>[6x]GSHMGTEDLKYSLERLREILERLEENPSEKQIVEAIRAIVENNAQIV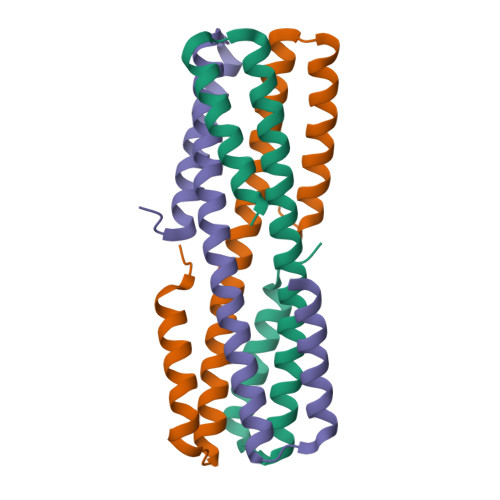EAIRAIVENNAQIVEILRAIIEALEAIGVDQKILEEMKKLLKDLKRSLERG Based on the structure-function knowledge of the RNase A superfamily we have engineered a chimera that combines RNase 1 highest catalytic activity with RNase 3 unique antipathogen properties. Based on the RNase 1 scaffold we incorporated specific regions essential for RNase 3 unique anti-pathogen activities within the RNase A superfamily. The solved crystal structures confirmed that all the chimera proteins reproduce the kidney-shaped folding typical of the RNase A superfamily and thus keep the fold of the templates used in their design, as suggested by circular dichroism and molecular dynamics analysis. Nonetheless, the structures that incorporated the key features related to RNase 3 antimicrobial activity retained the overall RNase 1 active site conformation together with the essential structural elements for binding to the human ribonuclease inhibitor (RNHI), ensuring non-cytotoxicity.

A first RNase hybrid construct was engineered to combine the high catalytic activity of human RNase 1 and the antimicrobial properties of RNase 3. Briefly, we incorporated the N-terminus of RNase 3 (1–45) that encompasses the main antimicrobial region of the protein and consists of the first two helices, which include an aggregation prone and a lipopolysaccharide (LPS) binding sequence. On the other hand, the hybrid construct conserved the flexible loop L1, ranging from residues 17 to 26 of RNase 1 and reported essential for the protein catalytic activity. A first construct (RNase 3/1-v1) was successfully designed with a catalytic activity 40-fold higher than RNase 3, but alas in detriment of its anti-pathogenic activity. The first version of RNase 3/1-v1 has twelve peptide chains in the asymmetric unit. The maximum RMSD deviation among backbone chains was 0.7, being the highest variation located within the last five C-terminal residues, suggesting that this region has a higher flexibility in solution. To note, the last beta strand was interrupted in residue Phe123, turning the C-terminal tail towards the active site cavity and, in particular, to the B2 region. We should also bear in mind that in the original RNase 1 structure the C-terminal beta strand includes two residues (Phe123 and Ser126) that are directly involved in the B1 cavity. Here, the location of these residues is displaced from their original position, suggesting an impact in the B1 base binding and selectivity, as later discussed. Surprisingly, the R1-L1 (D17-R27), predicted as highly flexible in RNase A studies, is here perfectly superposed between the twelve chains.

>MRPPQFTRAQWFAIQHIDSDSSPSSSSRYCTIAMRAINNYRWRCKPVNTFVHEPLVDVQNVCFQEKVTCKNGQGNCYRSRFRMHITDCRLTNGSKYPNCRYRTRPGRRHIIVACEGSPYVPVHFDASV[12x]>GSGGSGGITEAQARAIVNSALKLYSQDKTGMVDFALESGGGSILSTRCSETYETKTALMSLFGIPLWYFSQSPRVVIQPDIYPGNCWAFKGSQGYLVVRLSMMIHPAAFTLEHIPKTLSPTGNISSAPKDFAVYGLENEYQEEGQLLGQFTYDQDGESLQMFQALKRPDDTAFQIVELRIFSNWGHPEYTCLYRFRVHGEPVK[3x];>GSMTGQLFQKSVDAAPTQQEDSWTSLEHILWPFTRLRHNGPPPV[3x]

The Linker of Nucleoskeleton and Cytoskeleton (LINC) complex crosses both inner and outer nuclear membranes of the nuclear envelope to mechanically transduce cytoskeletal forces to nuclear contents. It is formed of nuclear SUN (Sad1 and UNC84 homology) and cytoplasmic KASH (Klarsicht, ANC-1, and Syne homology) proteins, which interact within the nuclear lumen. JAW1/LRMP (lymphoid restricted membrane protein) is an atypical KASH protein that is localised in the endoplasmic reticulum and outer nuclear membrane, and is specifically expressed in certain cells of the immune system, small intestine, pancreas and taste buds. Here, we report the crystal structure of the SUN-KASH complex between SUN1 and the non-canonical KASH domain of JAW1/LRMP (herein referred to as KASH6).

Thus, we crystallised the SUN1-KASH6 complex and solved its X-ray crystal structures from several crystals at resolutions between 1.7 and 2.3 Å. In contrast with previous SUN-KASH 6:6 structures, the SUN1-KASH6 crystal structure contains nine SUN domains, such that head-to-head interfaces of three SUN1 trimers interact together around a three-fold symmetry axis in a ‘trimer-of-trimers’ configuration. KASH6 peptides are clearly bound at both of these KASH-binding pockets of each SUN1 trimer (these are herein referred to as KASH6α and KASH6β). The third KASH-binding pocket of each SUN1 trimer is located on the underside of the trimer-of-trimers structure, away from inter-trimer interfaces. Here, we observed poor peptide electron density in the 1.7 Å resolution structure, and could build only three C-terminal KASH6 amino-acids (herein referred to as KASH6γ), with 71% occupancy. At the remaining KASH6γ/unbound site, KASH-lidγ adopts a low angled conformation in which its β-structure follows the path that would normally be occupied by the KASH peptide. This localisation likely acts as a steric hindrance for KASH-binding. As the only remaining binding interface is the minimal binding pocket for the KASH peptide C-terminus, this likely substantially reduces the binding affinity, accounting for the lack of stable binding by a third KASH6 peptide. Hence, treatment at pH 5.0 triggers the conformational change of SUN1-KASH6 from a symmetric head-to-head 6:6 structure into an asymmetric trimer-of-trimers 9:6 assembly. This conformational change requires the dissociation of two KASH6 molecules from each 6:6 complex. Hence, the few amino-acids of a KASH6γ peptide observed in the 1.7 Å crystal structure were likely remnants of the peptide having failed to fully dissociate upon trimer-of-trimers assembly.> DGVGNASGDWHCDSTWMGDRVVTKSTRTWVLPSYNNHQYREIKSGSVDGSNANAYFGYSTPWGYFDFNRFHSHWSPRDWQRLINNYWGFRPRSLRVKIFNIQVKEVTVQDSTTTIANNLTSTVQVFTDDDYQLPYVVGNGTEGCLPAFPPQVFTLPQYGYATLNRDNTENPTERSSFFCLEYFPSKMLRTGNNFEFTYNFEEVPFHSSFAPSQNLFKLANPLVDQYLYRFVSTNNTGGVQFNKNLAGRYANTYKNWFPGPMGRTQGWNLGSGVNRASVSAFATTNRMELEGASYQVPPQPNGMTNNLQGSNTYALENTMIFNSQPANPGTTATYLEGNMLITSES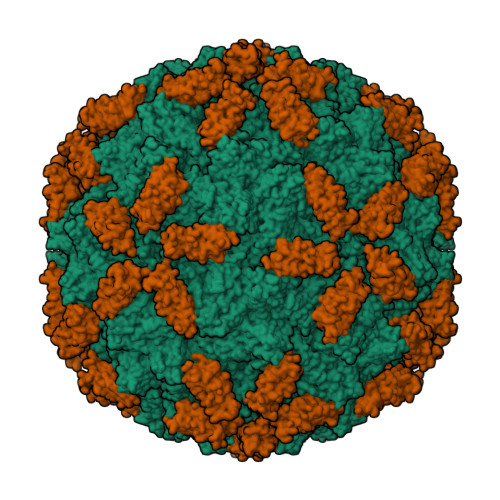ETQPVNRVAYNVGGQMATNNQSSTTAPATGTYNLQEIVPGSVWMERDVYLQGPIWAKIPETGAHFHPSPAMGGFGLKHPPPMMLIKNTPVPGNITSFSDVPVSSFITQYSTGQVTVEMEWELKKENSKRWNPEIQYTNNYNDPQFVDFAPDSTGEYRTTRPIGTRYLTRPL;> VIKELVVSAGESVQITLPKNEVQLNAYVLQEPPKGETYTYDWQLITHPRDYSGEMEGKHSQILKLSKLTPGLYEFKVIVEGQNAHGEGYVNVTVKPE>[2x]MNTRNPDKVVIVGGGTAGWMTASYLKKAFGERVSVTLVESGTIGTVGVGEATFSDIRHFFEFLDLREEEWMPACNATYKLAVRFQDWQRPGHHFYHPFEQMRSVDGFPLTDWWLQNGPTDRFDRDCFVMASLCDAGRSPRYLNGSLLQQEFDERAEEPAGLTMSEHQGKTQFPYAYHFEAALLAEFLSGYSKDRGVKHVVDEVLEVKLDDRGWISHVVTKEHGDIGGDLFVDCTGFRGVLLNQALGVPFVSYQDTLPNDSAVALQVPLDMEARGIPPYTRATAKEAGWIWTIPLIGRIGTGYVYAKDYCSPEEAERTLREFVGPEAADVEANHIRMRIG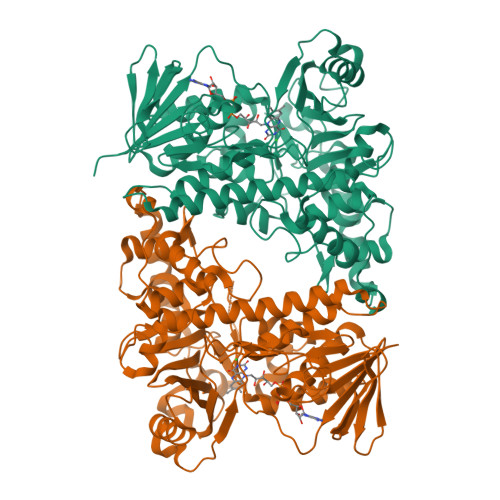RSEQSWKNNCVAIGLSSGFVEPLESTGIFFIHHAIEQLVKHFPAGDWHPQLRAGYNSAVANVMDGVREFLVLHYLGAARNDTRYWKDTKTRAVPDALAERIERWKVQLPDSENVFPYYHGLPPYSYMAILLGTGAIGLRPSPALALADPAAAEKEFTAIRDRARFLVDTLPSQYEYFAAMGQRV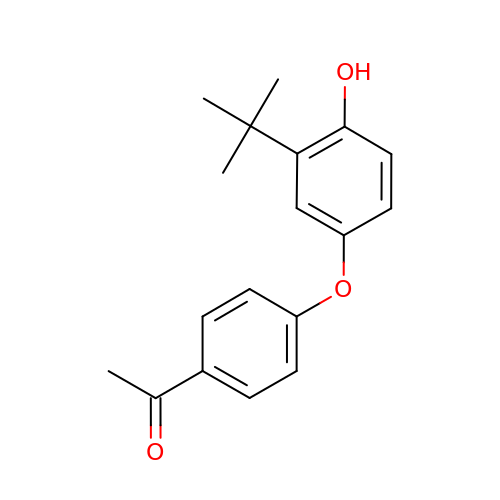1-[4-(3-tert-butyl-4-oxidanyl-phenoxy)phenyl]ethanone | C18 H20 O3 | WSVZSZVSZTYTCC-UHFFFAOYSA-N> MHHHHHHSSGRENLYFQGNKQWYLLANQLILSLSKYEGGHIFEKLVDAKKQNCPDYYDVIKNPMSFSCIKTKLKKGQYAYPSEFVKDVQLIFDNCSLYNTSNSVVAITGKNIETYFNNQLIVMGYNNFILKEKKINDMLKLVEEENIKWSKEKEDQIEEID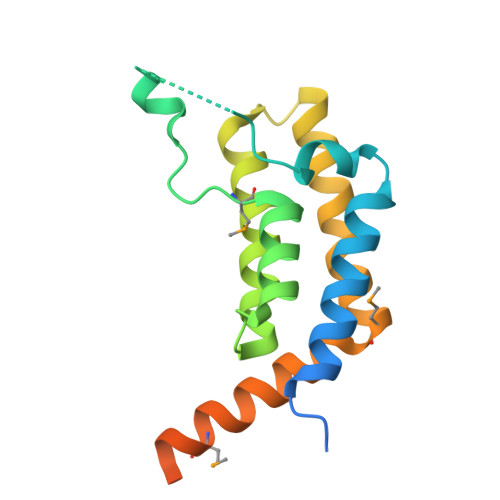ELENN> YEHTAVMPNKVGIPYKALVERPGYAPVHLQIQLVNTRIIPSTNLEYITCKYKTKVPSPVVKCCGATQCTSKPHPDYQCQVFTGVYPFMWGGAYCFCDTENTQMSEAYVERSEECSIDHAKAYKVHTGTVQAMVNITYGSVSWRSADVYVNGETPAKIGDAKLIIGPLSSAWSPFDNKVVVYGHEVYNYDFPEYGTGKAGSFGDLQSRTSTSNDLYA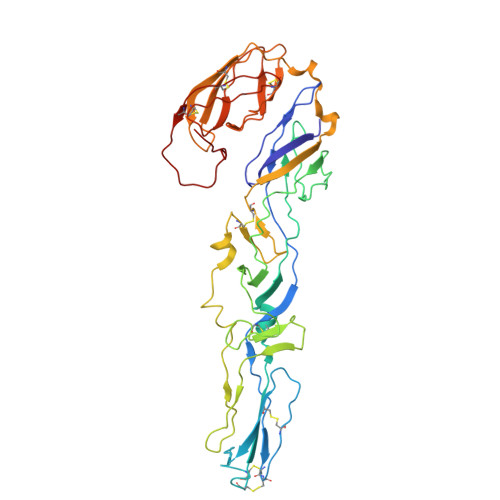NTNLKLQRPQAGIVHTPFTQAPSGFERWKRDKGAPLNDVAPFGCSIALEPLRAENCAVGSIPISIDIPDAAFTRISETPTVSDLECKITECTYASDFGGIATVAYKSSKAGNCPIHSPSGVAVIKENDVTLAESGSFTFHFSTANIHPAFKLQVCTSAVTCKGDCKPPKDHIVDYPAQHTESFT[(2~{R},3~{S},4~{S},5~{R})-3,4-bis(oxidanyl)-5-[3-[4-[[(phenylmethyl)amino]methyl]-1,2,3-triazol-1-yl]propyl]oxan-2-yl]methyl 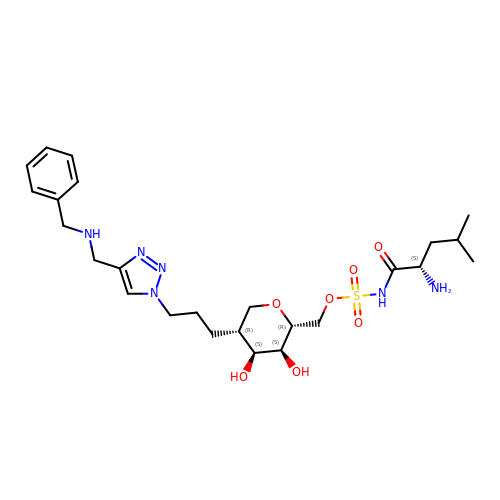~{N}-[(2~{S})-2-azanyl-4-methyl-pentanoyl]sulfamate | C25 H40 N6 O7 S | FOFGBZQNHMMVTL-MENZVKOBSA-N> ATAILRPIGLHVEKFQQTYRKKWRFLTSANANVILAEAASGERPARWALTTGMASIPWEYLFFYMSPAEYNRMKNYPGTFAKSASVRIRTWNTRVAFQTGDTQTANATLNQNKFLQVAKGIRSIPFICSTNRKYTYSDTEPMQPTGFATLTSYEYRDGLKTAMYGYDNDNKDFAKKPPADATGAEIYLQDYLTIYTNDARATTGTKILAGFPPYKNFIEEFDASACINTDVVAMDYDFSYAPLVPQFAPVPNNLITQNYNGSYPAGTKNEVTAAKTTDSSQATAPTQVRNAPRKYIQGPHADTTFFDEEQNYLRVPIEQGGIFEEV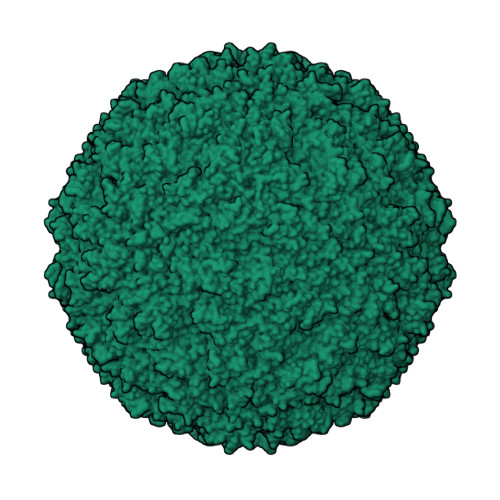NVETVHDTQMPSINVGIRAVPKLTTIDETTQANSWLDAQGYFEVDCVLTTESVDPYTYIKGGCYSANTKSQLQYFASDGRPIAKVYDNPNVYGRMQMIKTVKP>HMAQANFGVVGMAVMGKNLALNVESRGYTVAIYNRTTSKTEEVFKEHQDKNLVFTKTLEEFVGSLEKPRRIMLMVQAGAATDATIKSLLPLLDIGDILIDGGNTHFPDTMRRNAELADSGINFIGTGVSGGEKGALLGPSMMPGGQKEAYDLVAPIFEQIAAKAPQDGKPCVAYMGANGAGHYVKMVHNGIEYGDMQLIAESYDLLKRILGLSNAEIQAIFEEWNEGELDSYLIEITKEVLKRKDDEGEGYIVDKILDKAGNKGTGKWTSESALDLGVPLPLITESVFARYISTYKDERVKASKVLSGPALDFSGDKKEVIEKIRKALYFSKIMSYAQGFAQLRKASEEFDWDLPYGTIAQIWRAGCIIRAEFLQNITDAFDKDSELENLLLDDYFVDITKRYQEAVRDVVSLAVQAGTPIPTFTSAISYYDSYRSENLPANLIQAQRDYFGAHTYERTDKAGIFHYDWY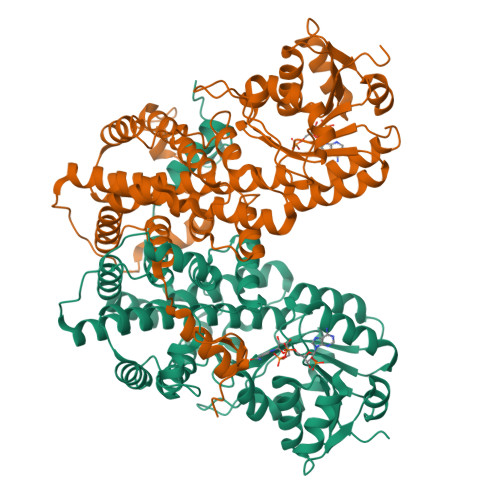TED[3x]4-[(~{E})-[3-(4-chlorophenyl)-5-sulfanylidene-1~{H}-1,2,4-triazol-4-yl]iminomethyl]benzoic 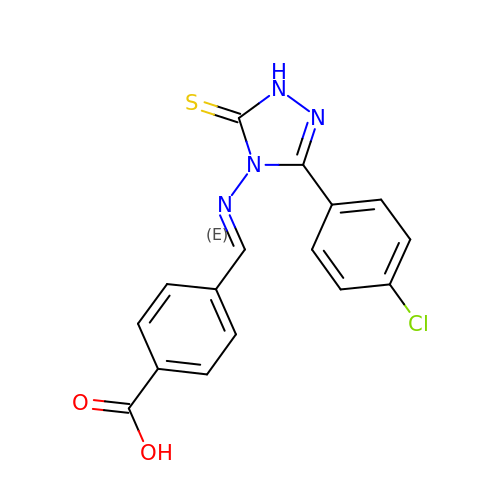acid | C16 H11 Cl N4 O2 S | CQVXUWVBXDJAGD-GIJQJNRQSA-N>[2x]MLNSFKLSLQYILPKLWLTRLAGWGASKRAGWLTKLVIDLFVKYYKVDMKEAQKPDTASYRTFNEFFVRPLRDEVRPIDTDPNVLVMPADGVISQLGKIEEDKILQAKGHNYSLEALLAGNYLMADLFRNGTFVTTYLSPRDYHRVHMPCNGILREMIYVPGDLFSVNHLTAQNVPNLFARNERVICLFDTEFGPMAQILVGATIVGSIETVWAGTITPPREGIIKRWTWPAGENDGSVALLKGQEMGRFKLG;>[2x]XTVINLFAPGKVNLVEQLESLSVTKIGQPLAVSTGHHHHHHG

Phosphatidylethanolamine (PE), a major component of the cellular membrane across all domains of life, is synthesized exclusively by membrane-anchored phosphatidylserine decarboxylase (PSD) in most bacteria. PSD is translated as an inactive proenzyme and undergoes self-cleavage between a conserved Gly-Ser pair to become an active αβ-heterodimer. This maturation step results in the post-translational modification of the N-terminus serine to pyruvoyl in the α-subunit, which is an indispensable prosthetic group for decarboxylation activity. After the proenzyme undergoes auto-proteolysis, an active complex is formed between the α- and β-chains, which are mainly responsible for catalytic activity and membrane association, respectively.

Using native and selenomethionine-derivatized recombinant PSD1–287, the crystal structures of apo PSD1–287 were determined from two crystal forms at resolutions of 1.90 and 2.63 Å, which are described as Apo-PSD1 and Apo-PSD2, respectively. The asymmetric unit of Apo-PSD1 contains two αβ-heterodimers, whereas that of Apo-PSD2 contains four. Two out of three molecules of N-dodecyl-b-maltoside (DDM), a detergent used to solubilize the enzyme, were located at the interface between two adjacent β-subunits, augmenting the dimerization of αβ-heterodimers in Apo-PSD1. Interestingly, DDM molecules identified in the structure of Apo-PSD1 interact with the positively charged surface of PSD through the relatively polar disaccharide moiety, whereas the dodecyl tail of the detergent interacts with the hydrophobic surface of the enzyme encompassing the N-terminal helices. These molecular interactions may mimic those occurring on the cellular membranes, where PSD is partially embedded within a single layer of phospholipids using the N-terminal helical domain. Estimation of the protein-membrane border in bacterial cells is further aided by co-crystallized DDM, the length of which roughly encompasses a single membrane leaflet. The N-terminal pyruvoyl residue (Pvl-254) of the α-subunit was unambiguously identified in both apo structures. Gly-253 of the β subunit, which is no longer connected to Pvl-254 after auto-cleavage, is approximately 12.6 Å apart when the distance between two Cαs is measured, and it forms a salt bridge with the side chain of Arg-221. Consequently, Pvl-254, which is located at the base of the funnel-shaped active site, is open for substrate binding.>MVTAAISGTDEIRARAEQALTRCGVDLTAVKGDALTARTPLTGADLFGLRAQTPEDVDRAVEAAHTAFLTWRTTPAPVRGALVKRFGELLTEHKQDLADLVTIEAGKIRSEALGEVQEMIDICDFAVGLSRQLYGRTMPTERPGHRLMETWHPLGVVGVISAFNF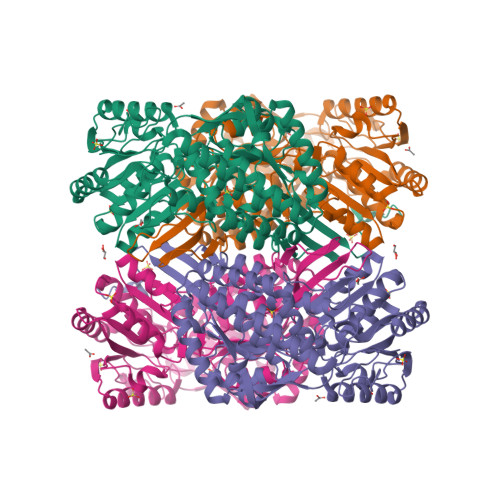PVAVWAWNAAVALVCGDTVVWKPSELTPLTALACAALLDLAIADAGAPKGLNQVVVGAADVGERLVDSPRVPLVSATGSTRMGRAVGPRVAARFGRTILELGGNNAAVVTPSADLDLTVNAAVFAAAGTAGQRCTTLRRLIVHEDIADTVVERLTAAFERLPIGDPFQDTTLVGPLVNEAAFGRMREAVERATAEGGTLCAGGERQFPDAAPGAYYVRPALVRMPAQTAVVREETFAPILYVLTYRDLDEAIRLNNEVPQGLSAGIFTADQSEAERFLAPDGADCGIANVNIGTSGAEIGGAFGGEKETGGGRESGSDAWRAYMRRATNTVNYSGRVTLAQGVDFSQ[2x]>[2x]HHHHHHFNLPPGNYKKPKLLYCSNGGHFLRILPDGTVDGTRDRSDQHIQLQLSAEGGGEVYIKSTETGQYLAMDTDGLLYGSQTPNEECLFLERLEENHYNTYISKKHAEKNWFVG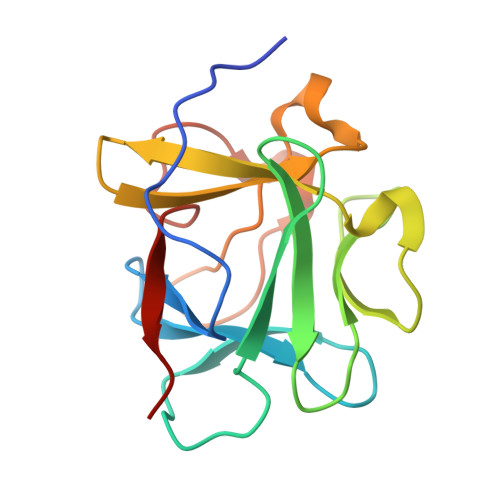LKKNGSCKRGPRTHYGQKAILFLPLPVSSD> MGVFRTRFTETFGVEHPIMQGG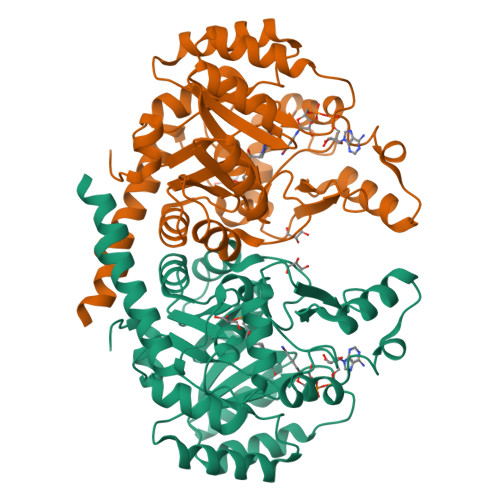MQWVGRAEMAAAVANAGGLATLSALTQPSPEALAAEIARCRELTDRPFGVNLTLLPTQKPVPYAEYRAAIIEAGIRVVETAGNDPGEHIAEFRRHGVKVIHKCTAVRHALKAERLGVDAVSIDGFECAGHPGEDDIPGLVLLPAAANRLRVPIIASGGFADGRGLVAALALGADAINMGTRFLATRECPIHPAVKAAIRAADERSTDLIMRSLRNTARVARNAISQEVLAIEARGGAGYADIAALVSGQRGRQVYQQGDTDLGIWSAGMVQGLIDDEPACAELLRDIVEQARQLVRQRLEGMLAGVHHHHHH The bacterial tight adherence pilus system (TadPS) assembles surface pili essential for adhesion and colonisation in many human pathogens. Pilus dynamics are powered by the ATPase CpaF (TadA), which drives extension and retraction cycles in Caulobacter crescentus through an unknown mechanism. We show that CpaF assembles into a hexamer with C2 symmetry in different nucleotide states. Nucleotide cycling occurs through an intra-subunit clamp-like mechanism that promotes sequential conformational changes between subunits.

To understand how the absence of nucleotide might regulate CpaF assembly and conformation, the structure of CpaF was determined by cryo-EM without nucleotide addition but in the presence of Mg2+. In this case, CpaF was less stable yielding a map resolved to 4.0 Å resolution overall. Henceforth, this CpaF structure obtained in the absence of nucleotide is termed CpaFAPO. CpaFAPO formed a C2 symmetric hexamer with subunits arranged in an open, closed and open’ conformation like CpaFAMPPNP and CpaFADP. No nucleotide or Mg2+ was observed in the nucleotide-binding pockets although HEPES was bound in the CTD/CTDn+1 clefts in both open and open’ state subunits. Superposition of the three distinct NTD2/CTDn+1 units within the CpaFAPO hexamer showed close alignment with RMSD Cα ≤ 0.7 Å. However, comparison of the CpaFAPO and CpaFADP asymmetric units showed that whilst similar, they do not pack identically and cannot be considered equivalent to CpaFADP superposed on CpaFAMPPNP. Specifically, Hinge 2 within the open state subunit is straightened so that its NTD2 moves towards the neighbouring NTD2 of the closed subunit. Consequently, the nucleotide-binding pocket in the open state subunit differs significantly in comparison to CpaFAMPPNP and CpaFADP as the associated NTD2/CTDn+1 unit has rotated. The overall effect is a relaxed and more rounded C2 symmetric hexamer.

>[6x]DYYHATKTTIFNALLNTIDLSQLAQLDLKQAGEEIRDIVAELVAIKNVSMSVAEQEHLVQDIINDVLGYGPLEPLLARDDIADIMVNGAHRVFIEVGGKVQLTNVRFRDNLQLMNICQRIVSQVGRRVDESSPICDARLPDGSRVNVIAPPLALDGPTLTIRKFKKDKLTMKNLVEFASISPEGARVLGVIGACRCNLVISGGTGSGKTTLLNTMTAFIDPTERVVTCEDAAELQLQQPHVVRLETRPPNLEGSGAVTMRDLVKNCLRMRPERIIVGEVRGPEAFDLLQAMNTGHDGSMGTLHANSPREAISRIESMITMGGYGLPSKTIKEMIVGSVDVIIQAARLRDGSRRITHITEVVGLEGDVIVTQDLFVYEITGEDEHGKVVGKHRSTGIARPRFWDRARYYGLERELAEALDAAEA> VILPNNNRHQIFNTTQGHYDAVSFIYIPIDGGYMSGSGVVVGENEILTNKHVVNGAKGNPRNISVHPSAKNENDYPNGKFVGQEIIPYPGNSDLAILRVSPNEHNQHIGQVVKPATISSNTDTRINENITVTGYPGDKPLATMWESVGKVVYIGGEELRYDLSTVGGNSGSPVFNGKNQVIGIHYGGVDNKYNSSVYINDFVQQFLRNNIPDINIQ

Staphylococcus epidermidis, a commensal of humans, secretes Esp protease to prevent Staphylococcus aureus biofilm formation and colonization. We show here that Esp cleaves autolysin (Atl)-derived murein hydrolases and prevents staphylococcal release of DNA, which serves as extracellular matrix in biofilms. The three-dimensional structure of Esp was revealed by x-ray crystallography and shown to be highly similar to that of S. aureus V8 (SspA). Iwase et al. reported that S. epidermidis Esp, a secreted serine protease, can disperse S. aureus biofilms.

Purified Esp was crystallized, and its three-dimensional structure was determined using x-ray crystallography. Esp displays a β-barrel fold assembled from two discrete domains and a C-terminal α-helix, similar to eukaryotic serine proteases of the chymotrypsin family. Even though Esp exhibits a highly conserved, compact β-barrel fold, the five or more intradomain disulfide bonds that are responsible for the structural rigidity of eukaryotic serine proteases are absent. Each of the two Esp domains is comprised of six antiparallel β-strands, and the solvent-accessible catalytic and substrate binding sites are situated at the interface of the two domains. In addition to the conserved position of putative catalytic triad residues (Ser235, Asp159, and His117), the substrate-binding region (S1 pocket) and the oxyanion hole, which together constitute the critical functional elements of activated serine proteases, are also conserved in Esp. The distances between Nϵ of the Esp active site His117 and Oγ of Ser235 and between Nδ of His117 and Oδ of Asp159 are 2.8 and 2.6 Å, respectively. The conformation of Ser235-Asn234-Gly233-Gly232-Val231 peptide segment in Esp is rigid with conserved backbone angles, supporting the presence of a functional oxyanion hole. Compared with all other eukaryotic serine proteases, loops 3 and D are absent in Esp and V8, and their loops 1 and 2 are also considerably shorter. Crystal structures of Esp and V8 display identical disposition for their N termini, which associate with respective S1 pockets more intimately than other active serine proteases. The N-terminal segment of Esp and V8 crosses over loop 1 into the bottom of the S1 pocket, and the N-terminal Val67 (V8 Val69) amino group is suitably positioned to act as an acceptor of the negative charge of P1 residue side chain.>[6x]MGSSHHHHHHSQDPLEVLFQGPEASMNLKPQTLMVAIQCVAARTRELDAQLQ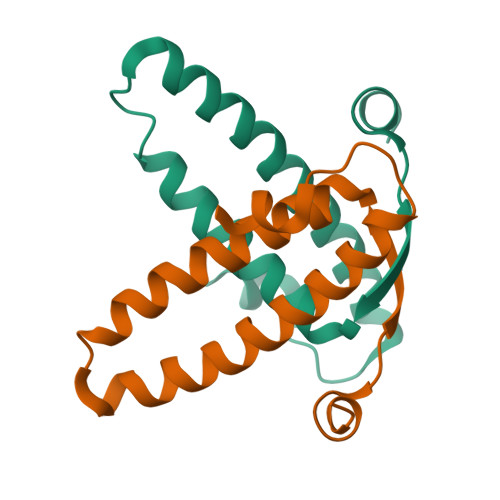NDDPQNAAELEQLLVGYDLAADDLKNAYEQALGQYSGLPPYDRLIEEPAS> LSPSSSPAKAQRTHLSLEEKIKLMRLVVRHKHEL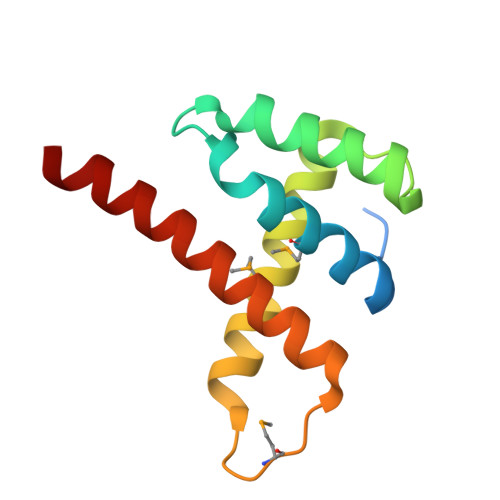VDRKTSEFYAKIARIGYEDEGLAIHTESACRNQIISIMRVYEQRLAHRQPGMKTTPEEDELDQLCDEWKARLSELQQYREKF>[2x]GSHMASLTEIEHLVQSVCKSYRETCQLRLEDLLRQRSNIFSREEVTGYQRKSMWEMWERCA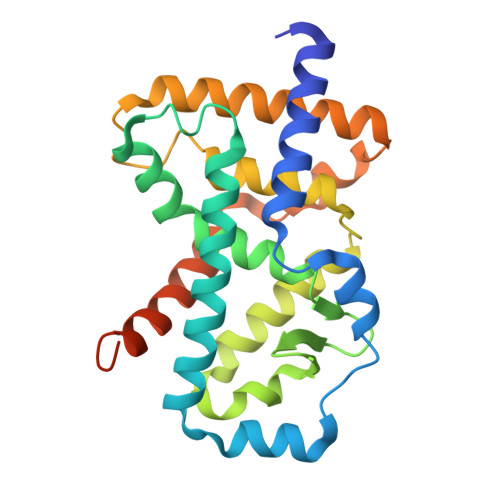HHLTEAIQYVVEFAKRLSGFMELCQNDQIVLLKAGAMEVVLVRMCRAYNADNRTVFFEGKYGGMELFRALGCSELISSIFDFSHSLSALHFSEDEIALYTALVLINAHRPGLQEKRKVEQLQYNLELAFHHHLCKTHRQSILAKLPPKGKLRSLCSQHVERLQIFQHLHPIVVQAAFPPLYKELFS> MKCSELWTEIIPKNDPNSNITNQVWSCSFNNDGSILLACVGDAILVYDSFTGNLVNKAIRGGQKEQINCIKFSKDGKRFATASNDKTVWVWSFDVNKNPKLAPEVKYSHTDKVLCLAFNPLTHQIFSGGAQDYALWTPDQQSIEKSKFKDKIITCAWSWDGLYLGFGTMGGIIGIRNRALEQLAEIQRSFPIWCMDWTPITPDYQNSVLVVGVWEQSIAHYNIQGQQLGSDKKLTYDPIDINFSTQGEFLLVSGTNNKCTLYTREGGFLIDVATKNDWVWNNKLKPVIKEAGSVAVQDQLHVALTTNDGEISMFKIQQLTVHALEGDKYAYRDNLTDIVVQSMSSNQRIRLKCKELVKNISIYKDKLAAHLTERILIYGTSSEDSQMKYKLHKRIVKKVEAHILEIVSNHLIACVKNKVQLYQLSGDLEKEWVFDSRVNCIKIIGGMPNKEGAYVGLKNGQIFKIFVDNSFPIPILNHNISIKNIDASQKRKRLAVVDKNSNLTVYDLSNKEQVFQEMNIVSCAFNNNFDDLLAFSSTDTTFIRCSNHPPLSQKISGQVVGFKANKLFVLNDNVMSTIDVSMTQTMIKYLERKEFQSAYEISLLGVTDQDFLYLGNEALIATQFAIARKCYTRIKKLDFIYLLEKAEKDFKKNTFVEGFYQGEIYALQTKFYEAENALTKSNLASQAKEMWIILKEFDKAMRITDTGASPINRGQNKEINSDASRKDLLIQRAEWEVKQGNWKKGGELYIQAEVYKKAIEVYVTNNFSEGIVEVCRNADAETQRKEIEQCAAYFKKAKLHQYTKEAYLKLQDNKALLQLNIDLEKWDEAMTLAKAHPEFMEIVKLPYANWLAKQDRYEESLKAYRKIGKHDMATKMLYNLSQNAVFEKRFSDAALFTWMIATEHLGLIRNMKAPTPEDIENLMKFYQYRDDAEIYFAYSKVQSFVDEPFLPLSGHAYMLNIFNAARFAINKLGNRQLYGVQHSYLYYSLGKVSKQLEGYKTARICYEKLASYKIPTEWSEEIELSTLLIRSKPYSDQESLLPICNRCYNQNPALTEGNRCSSCMHQFQNCFISFENLPLVEFKLDPKITHKRFIELINSDKSKTQPNKKKKKANDGWQESHQGDQQVLTFNNSPQKGGNDNESSPFLDKLNEVFEIQQTTQEYIPVTLDENIVSSLSIDEVYWVDYTKYCYTAEIKYYKSMLTDIPLKNCQECGTFYILDEYEFEISKTQKCPFCRSVDERAGPQKDVFDF;> MSLFSELPLDAGTDEQITQIAVSNVSINPSLAIITPHKILLFNECGEKHDYELSRNIRCTYVQWHPSQPIIALGWETGAITLWSEETKVAKEEPNGHKSEICLIQFNPSGSRMVSADIDGNVTVWRGINIVSQYKKEQSITHAIFCELNIDSKLKSGNLFFFGGKSGVVCLADDANHCSDVCKVGGSIKSLLFYEKENSVIIITSTLLLVMFKISTSVKTGPSKRVKLSISGDPQKLQSIWIGSCLLATCSHENMLRMWHLDQDDNYVLTLHQLAQQTQTQQGAATVIQSTNTNDQITSIQYEKRGKVLVAGTREGRIIFWKNLSIGSESPLDVDEWKMLPYVSVRQGVNSIAVGQNNGLIAVQYGNQISLVQETVINGKMTDQVRLLQSSANTIKIYINNDISNQVLHFQSKGNIKGLDCNDQFMLLWTSKTIEIHEIIINPKESQTKLVASIQEKCLRSVIHKENIILVNDMELNVLNFKGIQKQNLKFSESEGKILNVNVLNNHLIMWTSNNYIRLFDISRREVKQIGVTRRFENSQGQLGQIRYCAVNSDGSKIVITADQRGKSGPQADNKFYIYDVQTDNFLLYEMPAKCIPLQPYCDRKDRKFFGISCIINKNIQQEKNADENNDENEDNKSDKSRNEDDDEKDKSNLEFYTFFVTSENGIRKQDQYQLESSIEAVFAIDIPKLYFIKRNKKTNSSGQNYKIVEKYLNDFVGLEKIDNQIKEAIMNFSFYLTMDNLDEAYKSVKQIQNPSIWEKMASMCVKTKRIDVAEICLGNMRFARGSKAIREQKKEPELDAQLAMVAIQLNMKDEAVKLYEQSKRYDLYNKMLQAEGNWEKAIQISENHDRINLKNTYYRTAQMYEVSNNYEQAILYYEKSGTHVKEVPRMLLEAGQTEQLERYIIDKNEKPLFKWWAQYLESNYRIELAVKFYRQSEDYDQMVRLFLTKNDVQTASSICSETNNSAACYILAKYLEMNGQIPEAIQYYWKSQHYTQAVRLAREKGMDNEVMSISLQGPNQVKLQSAAYFEEKGFKQKAVELYKKGGNLIKAYNLAQEEKLYDEAKQIARQIEQEEDQRNKKRDPNDLAGIIDDFIEKGQPERAVPLMIKAKQFERAIETCIRFNIPITQDLVDKIIPTEPAKNAAEENKRKELMKLIADTSIKQGDYRLSSKLYTKLGNQVEAMKCLINLGAIDEVVNYATMARMPQLYILAGNFLQTTDWHKNPQLMKHIITFYNKAKAYDNLAGFFDACSSVEIDEYRDYEKAAAALNEALKHAKKSTSESRDFRIEQLETKLNLVQKFVQARALFSSDPQQMKQICEDLLAQPGIDQSVRSGDIYAQIIEYYYQVKNFSQAFDYIKKMQQKRIILAPYLDQEMLQQILESQGVSLNSKNKNNDDEFIEEDVPE;> MASSKKVFEFKDDLNGSGKVLFSWSQDCSYIAVCGQSKVVYVLDKRGRKLKETVLKSKNKVIGLEWDKDQEFLAILQENSTCFLLWNVFQNSFEQQDLEEKSKGSFIKWSKTHPVLVIGTEKGILYFYNKKTQKKIPTMGKHSKKITTGDWNDEGLLITGSEEKVLTVSSHNSDSKGESITVQHEPSNLQWARQKTDDRDSSQRTITAILSNKSILMYDLNTKKQPLELVYEPKYGKIVDYQLFGDGYIVTGFTEGYVAHVSSHLYELRDEIQSKRIFQSSLDALCTNDIIYKLAVAGENQIHIYNLGTWEEVKSQRIELPKAAGNVTKMQWANNGQLLVVATANGHLYGYLTSIPFLTSTYGSIVSVLSSFTEVSIVDTSRINQIQNVSSINLETEPGFLSLGLYHLAAGINNNVWYYLWLDQKRNGIIKGGEMIQKRDYLGSVKDIRLNEFWAAVLTDGKCILHTIQPNNNVKDQKFPQIETDKAISGIGLTNDFLIMLDSSGKIRYYHLEDQQFVVEYKPADCQLVKIYPNFSGTRVVCFDNKGSAYLFEPAQEQFYPLEHFPQRAEKVLWDQKDPNLFAVLQNDTLITFIINKNNINGTLIQPVKELLAIEDIKNPGPPVQTILDRGVKPLTLSNGLLKCFTPSGSINGQNLTSHSYLGSYKGRDDTDQGHYRFFLQNLQLHKYNNCLIAAQFLHNAVLYKELGRKALEFVDLDVALKSYQLAGSLSMVMTIQSFQHINEKNIIYGNIAMILGQYDLAQELFLKSSQPILALEMRSDIQDYLTALNLAKSIAPQEEPFICRRLAFQIENQGNNQEARKLYERAVLNKDDRPSDRSKIDNHNQLCFAGISRTSIKLGDIQRGVTIAKELIDNNIVIEIAVVCENMKQYLEAAELYQKSGMLEKAASLYIESKDFKKAAPLISMIKSPNLLKQYAKAKESEGAYNEAEQTYEQAESWEDVVRLNLDKLDNLRKAIAVLRTKCDTSTVCLMVANVCEKQGNYGELVEFLLKAGKKEEAFQKAQQYNVMDAYSDNMKDFTLEERLRIAQYYENQGIWVKAAKHFEQAKNPTKSLKLYLKAGDQYIDDMIDLVCRNKQQESLQQTLLDYLLEGEKPKDPIYLLKLYDKLGNIQSLVKIAITIASDEHDQGNYKIAHERLFETYQKVKEHNVAIPFDLEQKLMIIHSYILARKYLAYKEEDKEIELAAWLLNRVCKNISQFPTHAVNILTSAVIAAMKSKNRPLAYKWSVELVRPEYRSHINEKYKTRIENIARKPLKEEPVENKTECPFCKEYVGEFQLVCESCQNVIPFCIASGTHVIADQLCFCPSCRFPANINYFIKYAESEEGRCPMCSVQINLNEVKVENPEQAASILKQLRATRQSSEQKKK

Intraflagellar transport (IFT) trains, the polymers composed of two multi-subunit complexes, IFT-A and IFT-B, carry out bidirectional intracellular transport in cilia, vital for cilia biogenesis and signaling. The IFT-A complex is composed of six subunits (IFT144, IFT140, IFT122, IFT121, IFT139 and IFT43), mediating both the retrograde trafficking (toward the base) driven by the dynein-1b and the ciliary import of various membrane proteins across the ciliary gate. Here, we purified the IFT-A complex from protozoa Tetrahymena thermophila and determined the cryo-EM structures of the IFT-A complex and its subassemblies at a resolution range of 3.6 to 8.8 Å. Analysis of these structures reveal that the apo IFT-A complex is composed of two rigid structural modules, the head and base modules, and presents two distinct–elongated and folded states in solutions, the latter of which was not identified in recent IFT-A structural studies.

In particular, IFT144, IFT140, IFT122 and IFT121, share the same domain organization, from the N- to the C-termini encompassing two tandem WD40 β-propellers (WDs), an array of 12 to 20 TPRs and, except for IFT140, a zinc binding domain (ZBD). These four subunits are distributed into the two modules; the head module consists of IFT140, IFT144 and the C-terminal half of IFT122 (IFT122C, 706-1246), whereas the base module consists of IFT121, the N-terminus of IFT122 (IFT122N, 1-705) as well as IFT139 and IFT43. Intriguingly, the N-terminal WD40 propellers together with the first four TPRs of both IFT140 and IFT144 in the head module are organized by pseudo-two-fold symmetry, in which a unique α-helical insertion between the second and the third TPRs in IFT140 and IFT144 allows TPRs at the junction to lock into a zigzagged configuration in both shape and electrostatic complementary manners. In the head module, the ~15-residue linkers between the second WD40 propeller and the first TPR in both IFT140 and IFT144 make a sharp turn such that the propellers of IFT140 and IFT144 point to opposite directions away from the central pseudo-two-fold axis in an elongated conformation. The C-terminal ZBD of IFT122 attaches to the other side of the IFT140-IFT144 TPR junction to constitute a compact core that is further encircled by the TPR array of IFT140, burying a total of ~2500 Å2 solvent exposed surface area. From this core extend out the TPR arms of IFT122, IFT140 and IFT144, the most variable segments in the head module. A frameshift mutation at Tyr1077 in human IFT122ZBD (equivalent to Lys1013 in Tetramymena IFT122ZBD) that would disrupt the head module core causes the severe Beemer-Langer syndrome with early infant death or Cranioectodermal dysplasia, highlighting the essential role of IFT122ZBD in organizing the head module core in IFT-A. Structural comparison shows that individual head and base modules are almost identical in these two states.>MASMTGGQQMGRGSAGVLPAHGTQHGIRLPLRSGLGGAPLGLRLPRETDEEPEEPGRRGSFVEMVDNLRGKSGQGYYVEMTVGSPPQTLNILVDTGSSNFAVGAAPHPFLHRYYQRQLSSTYRDLRKGVYVPYTQGKWEGELGTDLVSIPHGPNVTVRANIAAITESDKFFINGSNWEGILGLAYAEIARPDDSLEPFFDSLVKQTHVPNLFSLQLCGAGFPLNQSEVLASVGGSMIIGGIDHSLYTGSLWYTPIRREWYYEVIIVRVEINGQDLKMDCKEYNYDKSIVDSGTTNLRLPKKVFEAAV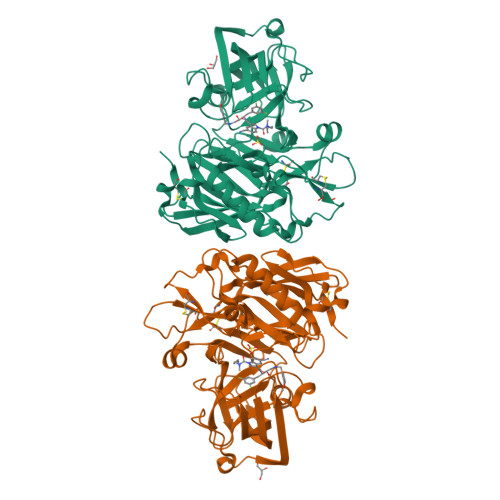KSIKAASSTEKFPDGFWLGEQLVCWQAGTTPWNIFPVISLYLMGEVTNQSFRITILPQQYLRPVEDVATSQDDCYKFAISQSSTGTVMGAVIMEGFYVVFDRARKRIGFAVSACHVHDEFRTAAVEGPFVTLDMEDCGYNIPQTDEST[2x]> GSGHACYRNCWR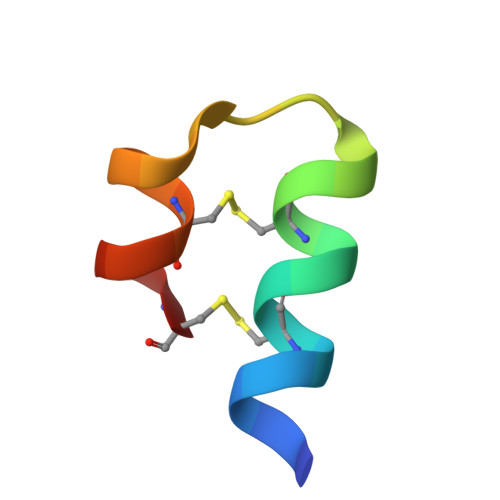EGNDEETCKERCG>GSHMALLVEKTTSGREYKVKDMSQADFGRLEIELAEVEMPGLMASRSEFGPSQPFKGAKITGSLHMTIQTAVLIETLTALGAEVRWCSCNIFSTQDHAAAAIARDSAAVFAWKGETLQEYWWCTERALDWGPGGGPDLIVDDGGDTTLLIHEGVKAEEIYEKSGQFPDPDSTDNAEFKIVLSIIKEGLKTDPKRYHKMKDRVVGVSEETTTGVKRLYQMQANGTLLFPAINVNDSVTKSKFDNLYGCRHSLPDGLMRATDVMIAGKVAVVAGYGDVGKGCAAALKQAGARVIVTEIDPICALQATMEGLQVLTLEDVVSEADIF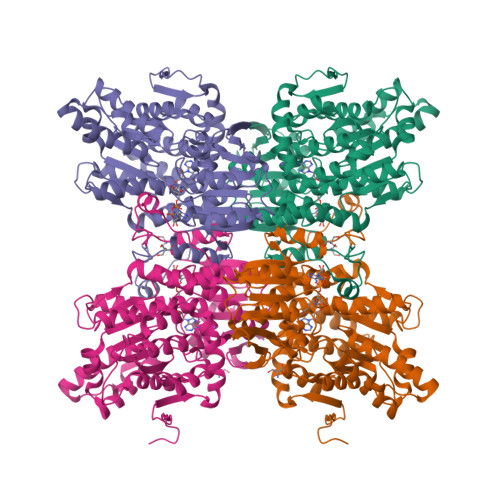VTTTGNKDIIMLDHMKKMKNNAIVCNIGHFDNEIDMLGLETHPGVKRITIKPQTDRWVFPETNTGIIILAEGRLMNLGCATGHPSFVMSCSFTNQVIAQLELWNEKSSGKYEKKVYVLPKHLDEKVAALHLEKLGAKLTKLSKDQADYISVPVEGPYKPFHYRY[2x]>[4x]MHHKAKVIGMLKETIRSGDWKGEKHVPVIEYEREGDLVKVEVSV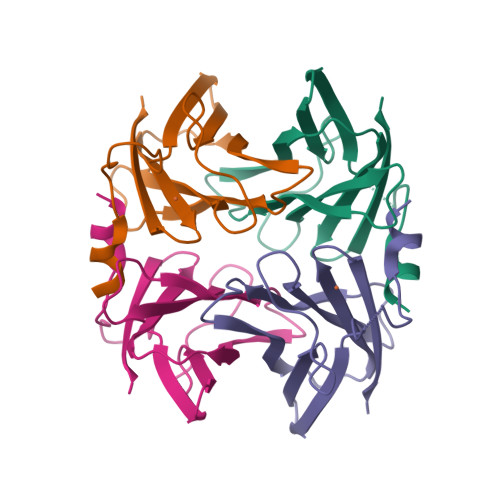GKEIPHPNTPEHHIAWIELYFHPEGGQFPILVGRVEFTNHSDPLTEPRAVFFFKTSKKGKLYALSYCNIHGLWENEVQLE>ACVFFCEDAA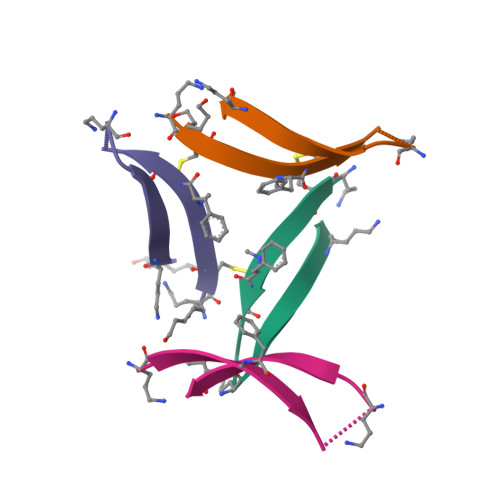VIGLAV[4x]The CysN polypeptide also contains a C-terminal APS (adenosine-5’-phosphosulfate) kinase domain (CysC), which exists as a separate enzyme in other bacteria and plants. Alternatively, APS can be phosphorylated at the 3′-position by APS kinase (CysC) to generate 3′-phosphoadenosine 5′-phosphosulfate (PAPS), a substrate for sulfotransferases that catalyze the transfer of the sulfate group onto a variety of metabolites. The structure of CysC is characterized by the canonical α/β-purine nucleotide binding fold, consisting of a five-stranded parallel β-sheet which is flanked on both sides by two α-helices. Structural features typical of APS kinases of this fold family, including the P-loop required for ATP binding (residues 452–458 in CysC), the conserved LDGD motif (residues 477–480) and the lid region (residues 552–581) above the P-loop which closes upon substrate binding, are also found in CysC.

To obtain more insights into the active site of CysC from M. tuberculosis and modes of ligand binding, we co-crystallized CysC in the presence of ADP, APS and Mg2+ and determined the structure of this complex. The overall structure of the CysC protein core and the subunit-subunit interface in the ternary complex CysC•ADP•APS is similar to the structure of the binary complex CysC•ADP. Superimposition of the individual subunits resulted in an rmsd of 0.9 Å. This relatively high value is, however, due to the shift of one loop in response to APS binding. In the ternary complex ADP is bound in a well-defined conformation in the canonical nucleotide binding site in the vicinity of the P-loop and the enzyme-ADP interactions are well preserved compared to the binary complex. We note, however, that in spite of the presence of 2 mM Mg2+ during crystallization no electron density indicating a bound Mg2+ ion is observed in the vicinity of the diphosphate group. The APS adenine ring is sandwiched between Phe492 and Phe576 in a π-stacking arrangement, an interaction conserved in other complexes of APS kinase. The phosphate group interacts with the side chain of Arg483 and the main chain nitrogen atom of Ile523 and the sulfate group forms hydrogen bonds to the side chains of Arg483 and Arg497 and the main chain nitrogen atom of Ser524. However, we observe this shift in position of helix α5 already in the CysC•ADP•APS complex, i.e. in the absence of Mg2+, implying that APS binding rather than binding of the metal ion triggers this structural re-arrangement in CysC.

>PPRGKTVWFTGLSGSGKSSVAMLVERKLLEKGISAYVLDGDNLRHGLNADLGFSMADRAENLRRLSHVATLLADCGHLVLVPAISPLAEHRALARKVHADAGIDFFEVFCDTPLQDCERRDPKGLYAKARAGEITHFTGIDSPYQRPKNPDLRLTPDRSIDEQAQEVIDLLES[2x]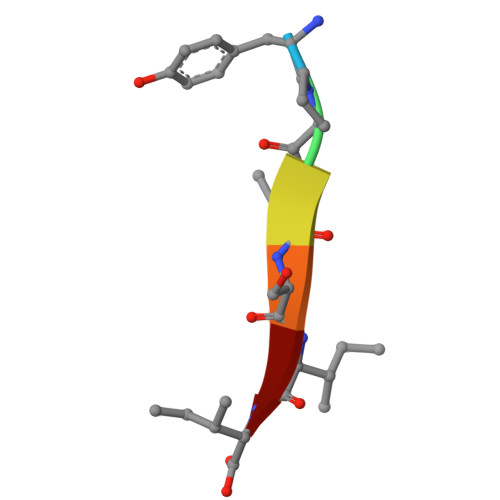> YPTSII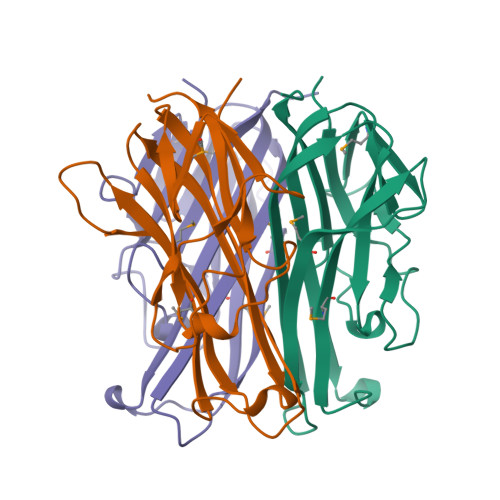>GKPEAQPFAHLTINAASIPSGSHKVTLSSWYHDRGWAKISNMTLSNGKLRVNQDGFYYLYANICFRHHETSGSVPTDYLQLMVYVVKTSIKIPSSHNLMKGGSTKNWSGNSEFHFYSINVGGFFKLRAGEEISIQVSNPSLLDPDQDATYFGAFKVQDID[3x]>MGNAQERPSETIDRERMRLVETLQADSGLLLDALLARGVLTGPEYEALDALPDAERRVRRLLLLVQGKGEAACQELLRCAQRTAGAPDPAWDWQH[2x]

Apoptosis repressor with caspase recruiting domain (ARC) is a multifunctional modulator of apoptosis. Human ARC contains 208 amino acids and is composed of two distinct domains, N-terminal caspase recruiting domain (CARD) domain and C-terminal P/E (proline and glutamic acid) rich domain. ARC is a unique apoptosis inhibitor in that it can antagonize both the intrinsic and extrinsic pathways. ARC CARD interacts directly with the death domains (DD) of Fas and FADD, as well as with the death effector domains (DEDs) of procaspase-829.

To better understand the CARD domain-mediated inhibition mechanism of ARC during apoptosis signaling, we report the first crystal structure of the CARD domain of ARC containing amino acids 1–95 at a resolution of 2.4 Å. The high resolution structure of ARC CARD showed that it comprises five helices, H1 to H5, which is not the typical fold of the DD superfamily. Interestingly, the sixth helix (H6) was not detected at the typical location, indicating that H6 might be flexible in the CARD domain of ARC or adopt a loop structure instead. There were two monomers in the asymmetric unit, chain A and chain B. The model of chain A was built from residue 5 to residue 87 and residue 91 to residue 93, while that of chain B was built from residue 5 to residue 84. The helix bundle from H1 to H5 was tightly packed by a central hydrophobic core composed of I12, V20, L23, L30, L31, L34, L35, L40, L48, V58, L61, L62, L64, V65, L76, and L77. The two ARC CARDs in the asymmetric unit are packed as an asymmetric dimer with an interface composed primarily of an electrostatic interaction. The principal interaction forces are salt bridges and hydrogen bonds, which are made by D13 (on H1), R56 (on H4), R59 (on H4), and R60 (H4) from chain A and by D32 (on H2), R37 (on H2), E46 (on H3), and D49 (on H3) from chain B. Although a unique disulfide bond-mediated homo-dimeric structure of the CARD domain including NOD1 and CARMA1 has been reported, the current structure of ARC CARD was dimerized via a Type I interface, which is a novel method for the homo-dimeric CARD structure. The size exclusion chromatography and MALS experiment showed that the dimeric ARC CARD became a monomer via mutations of interface residue D49R, R56E, and R59E, and double mutants.>[2x]GSHMRY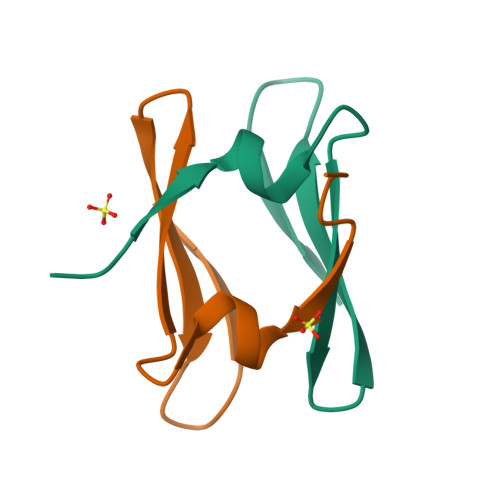TDSRKLTPETDANHKTASPQPIRRISSQTLLGPDGKLIIDHDGQEYLLRKTQAGKLLLTK> QVPSD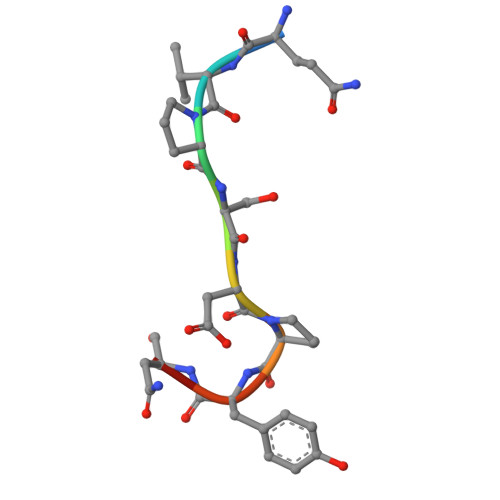PYNY>MMKILNSFSLKPEQRQTLEAAGHTVIDADKLDDATAQQIDVVYGWNAAATRVNFDRLQFVQAMSAGVDYLPLAELAKHHVLLANTSGIHAEPIAEYVLGALFTISRGILPAIRADRDMWTLRQERPPMTLLKGKTA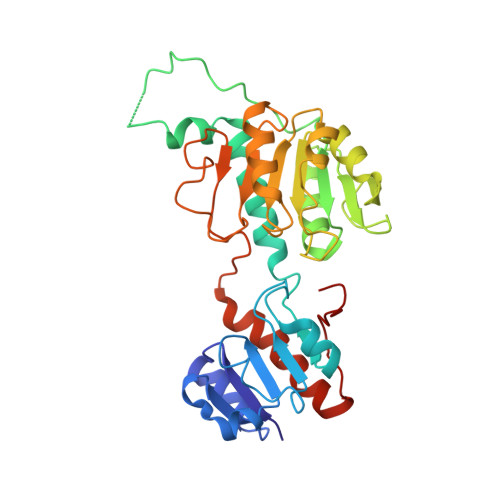VIFGTGHIGSTIATKLQALGLHTIGVSAHGRPAAGFDQVMTDVATHEAAGRADVVINALPLTPDTKHFYDEAFFAAASKQPLFINIGRGPSVDMAALTQALKNKQISAAALDVVDPEPLPQDSPLWGMTNVLLTPHISGTVPQLRDKVFKIFNDNLKTLISSGQLASHQVDLTRGY[2x]> MNTYFDIPHRLVGKALY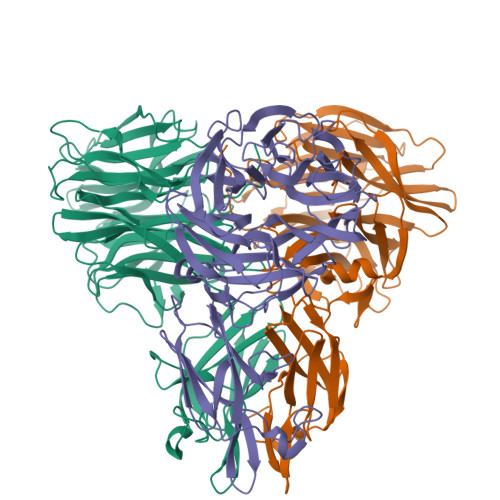ESYYDHFGQMDILSDGSLYLIYRRATEHVGGSDGRVVFSKLEGGIWSAPTIVAQAGGQDFRDVAGGTMPSGRIVAASTVYETGEVKVYVSDDSGVTWVHKFTLARGGADYNFAHGKSFQVGARYVIPLYAATGVNYELKWLESSDGGETWGEGSTIYSGNTPYNETSYLPVGDGVILAVARVGSGAGGALRQFISLDDGGTWTDQGNVTAQNGDSTDILVAPSLSYIYSEGGTPHVVLLYTNRTTHFCYYRTILLARAVAGSSGWTERVPAYSAPAASGYTSQVVLGGRRILGNLFRETSSTTSGAYQFEVYLGGVPDFESDWFSVSSNSLYTLSHGLQRSPRRVVVEFARSSSPSTWNIVMPSYFNDGGHKGSGAQVEVGSLNIRLGTGAAVWGTGYFGGIDNSATTRLATGYYRVRAWI(2R)-3-(4-hydroxyphenyl)-2-{[(2E)-3-(4-hydroxyphenyl)prop-2-enoyl]oxy}propanoic acid | C18 H16 O6 | 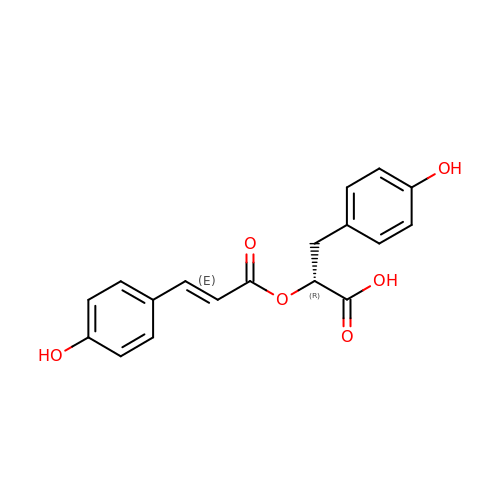LVPGCTXCBGXZHO-ZWIJEDICSA-N>[3x]TTGHSYEKYNNWETIEAWTKQVTSENPDLISR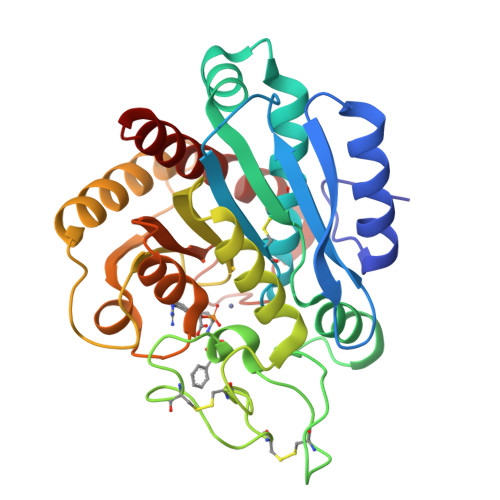TAIGTTFLGNNIYLLKVGKPGPNKPAIFMDCGFHAREWISHAFCQWFVREAVLTYGYESHMTEFLNKLDFYVLPVLNIDGYIYTWTKNRMWRKTRSTNAGTTCIGTDPNRNFDAGWCTTGASTDPCDETYCGSAAESEKETKALADFIRNNLSSIKAYLTIHSYSQMILYPYSYDYKLPENNAELNNLAKAAVKELATLYGTKYTYGPGATTIYPAAGGSDDWAYDQGIKYSFTFELRDKGRYGFILPESQIQATCEETMLAIKYVTNYVLGHL> MSSRYLLSPAAQAHLEEIWDCTYDRWGVDQAEQYLRELQHAIDRAAANPRIGRACDEIRPG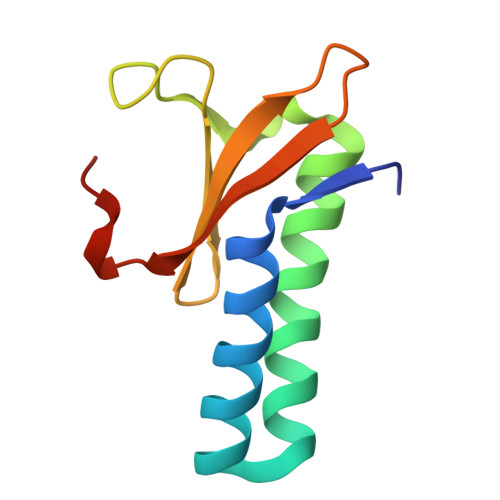YRKLSAGSHTLFYRVTGEGTIDVVRVLHQRMDVDRNL> MSRYFKVTACIPSLKRVRTGRELQ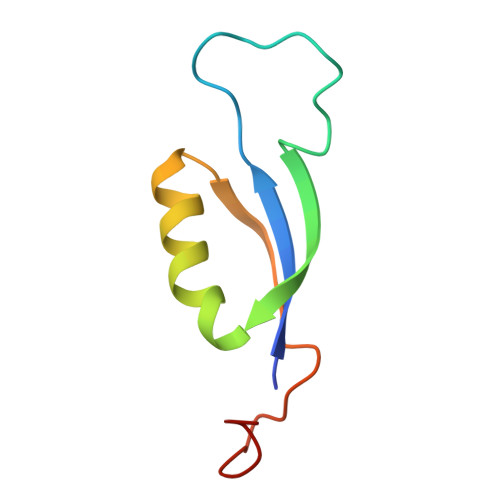NTFFTKLVPYENWFTEQQRIQKAGGKVLSVKLFTGVQGANTGVGA>KKNTAASLQQWKVGDKCSAIWSEDGCIYPATIASIDFKRETCVVVYTGYGNREEQNLSDLLSPICE[4x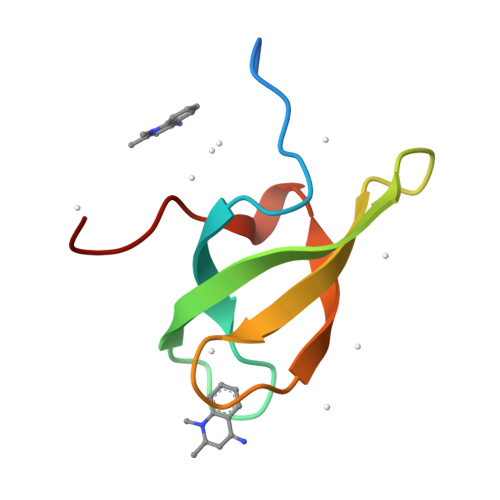]>GPGSKPQEPATAEIKPNKKILIELKVEKKPMGVIVCGGKNNHVTTGCVITHVYPEGQVAADKRLKIFDHICDINGTPIHVGSMTTLKVHQLFHTTYEKAVTLTVFRADPPELEKFNVDLMKKAGKELGLSLSPNEIGCTIADLIQGQYPEIDSKLQRGD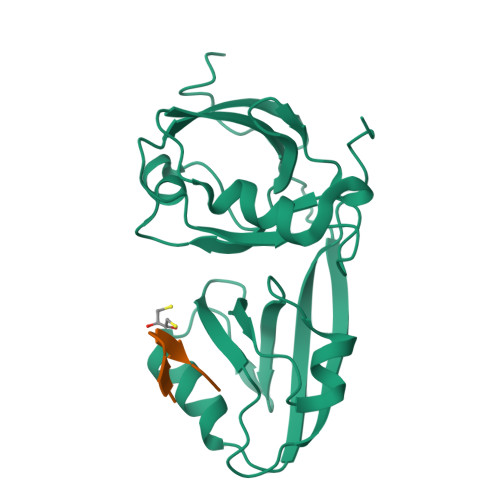IITKFNGDALEGLPFQVCYALFKGANGKVSMEVTRPKPTLRTEAPKA[8x];>[8x]ALRNGQYWV>[2x]GAQQQELPVPKPHQLKWHEAEMGAVFHYDLHVFDGIRYGQGNNRINPIEDYNIFNPTELNTDQWVQAAKAAGCKFAVLTATHETGFGLWQSDVNPYCLKAVKWRDGKGDIVRDFVNSCRKYGLQPGIYIGIRWNSLLGIHNFKAEGEGAFARNRQAWYKRLCEKMVTELCTRYGDLYMIWFDGGADDPRADGPDVEPIVNKYQPNCLFYHNIDRADFRWGGSETGTVEYPCWSTF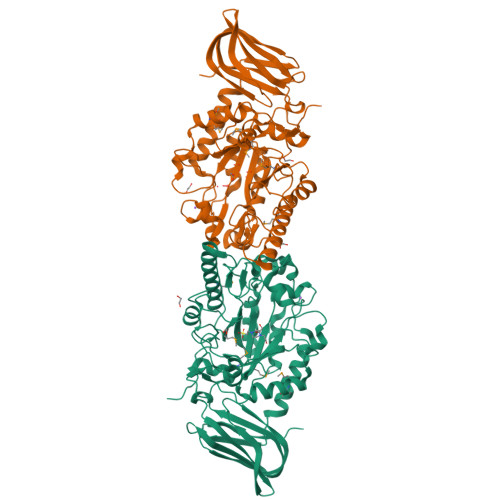PVPCSHHKRIESSIDQLELLKHGDKNGRYWVPAMADTPLRGANGRHEWFWEPDDENNIYPLNTLMDKYEKSVGRNATLILGLTPDPTGLIPAGDAQRLKEMGDEINRRFSSPIARISGQKKSLTLKLGKEQSVNYCIIQENIKNGERIRQYQIEAKVNGKWQTVCKGESVGHKRIEKFEPVEATALRLTVSESIALPDIINFSAYSVK>MNDLNVLVLEDEPFQRLVAVTALKKVVPGSILEAADGKEAVAILESCGHVDIAICDLQMSGMDGLAFLRHASLSGKVHSVILSSEVDPILRQATISMIECLGLNFLGDLGKPFSLERITALLTRYNARRQDLPRQIEVAELPSVADVVRGLDNGEFEAYYQPKVALDGGGLIGAEVLARWNHPHLGVLPPSHFLYVMETYNLVDKLFWQLFSQGLATRRKLAQLGQPINLAFNVHPSQLGSRALAENISALLTEFHLPPSSVMFEITETGLISAPASSLENLVRLWIMGCGLAMDDFGAGYSSLDRLCEFPFSQI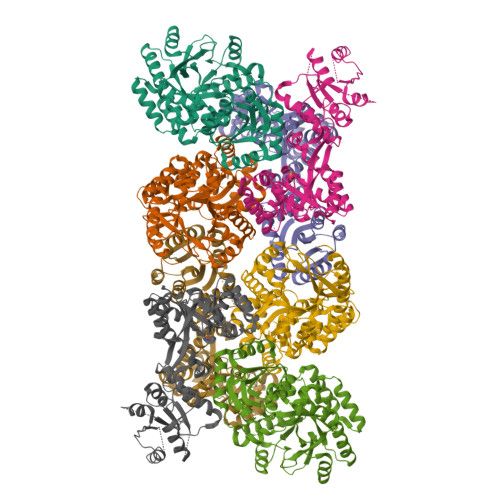KLDRTFVQKMKTQPRSCAVISSVVALAQALGISLVVEGVESDEQRVRLIELGCSIAQGYLFARPMPEQHFLDYCSGSLEHHHHHH[4x]>[2x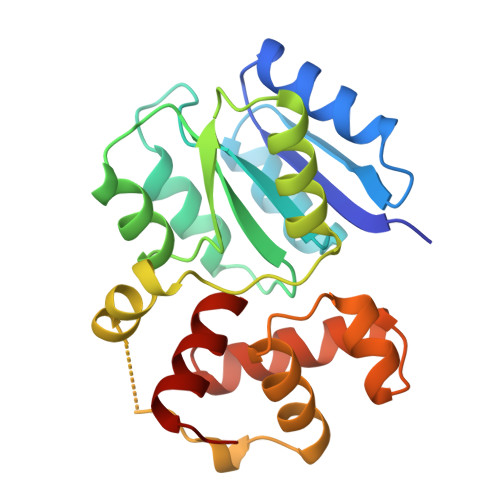]SNQEPATILLIDDHPMLRTGVKQLISMAPDITVVGEASNGEQGIELAESLDPDLILLDLNMPGMNGLETLDKLREKSLSGRIVVFSVSNHEEDVVTALKRGADGYLLKDMEPEDLLKALHQAAAGEMVLSEALTPVLAASLRANRATTERDVNQLTPRERDILKLIAQGLPNKMIARRLDITESTVKVHVKHMLKKMKLKSRVEAAVWVHQERIF> MAVDSAMELLFLDTFKHPSAEQSSHIDVVRFPCVVYINEVRVIPPGVRAHSSLPDNRAYGETSPHTFQLDLFFNNVSKPSAPVFDRLGSLEYDENTSIIFRPNSKVNTDGLVLRGWYNCLTLAIYGSVDRVISHDRDSPPPPPPPPPPPQPQPSLKRNPKHADGEKEDQFNGSPPRPQPRGPRTPPGPPPPDDDEDDPVPLPVSGDKEEDAPHREDYFEPISPDRNSVPQEGQYSDEGEVEEEQQEEGEEDEDDVDVEEEEDEDEDDRRTVDSIPEEEEEDEEEEGEEDEEGEGDDGYEQISSDEDGIADLERETFKYPNFDVEYTAEDLASVPPMTYDPYDRELVPLLYFSCPYKTTFEIEISRMKDQGPDKENSGAIEASVKLTELLDLYREDRGAKWVTALEEIPSLIIKGLSYLQLKNTKQDSLGQLVDWTMQALNLQVALRQPIALNVRQLKAGTKLVSSLAECGAQGVTGLLQAGVISGLFELLFADHVSSSLKLNAFKALDSVISMTEGMEAFLRGRQNEKSGYQKLLELILLDQTVRVVTAGSAILQKCHFYEVLSEIKRLGDHLAEKTSSLPNHSEPDHDTDAGLERTNPEYENEVEASMDMDLLESSNISEGEIERLINLLEEVFHLMETAPHTMIQQPVKSFPTMARITGPPERDDPYPVLFRYLHSHHFLELVTLLLSIPVTSAHPGVLQATKDVLKFLAQSQKGLLFFMSEYEATNLLIRALCHFYDQDEEEGLQSDGVIDDAFALWLQDSTQTLQCITELFSHFQRCTASEETDHSDLLGTLHNLYLITFNPVGRSAVGHVFSLEKNLQSLITLMEYYSKEALGDSKSKKSVAYNYACILILVVVQSSSDVQMLEQHAASLLKLCKADENNAKLQELGKWLEPLKNLRFEINCIPNLIEYVKQNIDNLMTPEGVGLTTALRVLCNVACPPPPVEGQQKDLKWNLAVIQLFSAEGMDTFIRVLQKLNSILTQPWRLHVNMGTTLHRVTTISMARCTLTLLKTMLTELLRGGSFEFKDMRVPSALVTLHMLLCSIPLSGRLDSDEQKIQNDIIDILLTFTQGVNEKLTISEETLANNTWSLMLKEVLSSILKVPEGFFSGLILLSELLPLPLPMQTTQVIEPHDISVALNTRKLWSMHLHVQAKLLQEIVRSFSGTTCQPIQHMLRRICVQLCDLASPTALLIMRTVLDLIVEDLQSTSEDKEKQYTSQTTRLLALLDALASHKACKLAILHLINGTIKGDERYAEIFQDLLALVRSPGDSVIRQQCVEYVTSILQSLCDQDIALILPSSSEGSISELEQLSNSLPNKELMTSICDCLLATLANSESSYNCLLTCVRTMMFLAEHDYGLFHLKSSLRKNSSALHSLLKRVVSTFSKDTGELASSFLEFMRQILNSDTIGCCGDDNGLMEVEGAHTSRTMSINAAELKQLLQSKEESPENLFLELEKLVLEHSKDDDNLDSLLDSVVGLKQMLESSGDPLPLSDQDVEPVLSAPESLQNLFNNRTAYVLADVMDDQLKSMWFTPFQAEEIDTDLDLVKVDLIELSEKCCSDFDLHSELERSFLSEPSSPGRTKTTKGFKLGKHKHETFITSSGKSEYIEPAKRAHVVPPPRGRGRGGFGQGIRPHDIFRQRKQNTSRPPSMHVDDFVAAESKEVVPQDGIPPPKRPLKVSQKISSRGGFSGNRGGRGAFHSQNRFFTPPASKGNYSRREGTRGSSWSAQNTPRGNYNESRGGQSNFNRGPLPPLRPLSSTGYRPSPRDRASRGRGGLGPSWASAN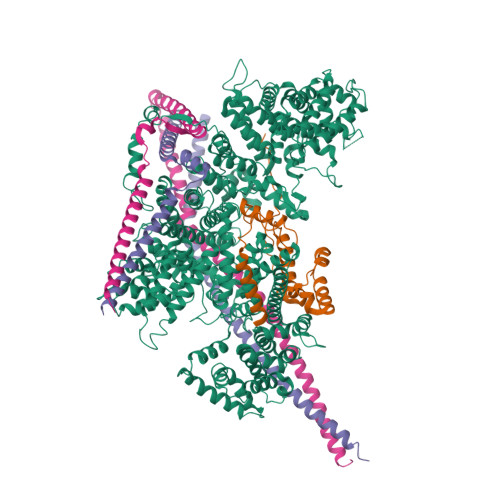SGSGGSRGKFVSGGSGRGRHVRSFTR;> PVATATATTVPATLAATTAAAATSFSTSAITISTSATPTNTTNNTFANEDSHRKCHRTRVEKVETPHVTIEDAQHRKPMDQKRSSSLGSNRSNRSHTSGRLRSPSNDSAHRSGDDQSGRKRVLHSGSRDREKTKSLEITGERKSRIDQLKRGEPSRSTSSDRQDSRSHSSRRSSPESDRQVHSRSGSFDSRDRLQERDRYEHDRERERERRDTRQREWDRDADKDWPRNRDRDRLRERERERERDKRRDLDRERERLISDSVERDRDRDRDRTFESSQIESVKRCEAKLEGEHERDLESTSRDSLALDKERMDKDLGSVQGFEETNKSERTESLEGDDESKLDDAHSLGSGAGEGYEPISDDELDEILAGDAEKREDQQDEEKMPDPLDVIDVDWSGLMPKHPKEPREPGAALLKFTPGAVMLRVGISKKLAGSELFAKVKETCQRLLEKPKDADNLFEHELGALNMAALLRKEERASLLSNLGPCCKALCFRRDSAIRKQLVKNEKGTIKQAYTSAPMVDNELLRLSLRLFKRKTTCHAPGHEKTEDNKLSQSSIQQELCVS;>[2x]MTNEEPLPKKVRLSETDFKVMARDELILRWKQYEAYVQALEGKYTDLNSNDVTGLRESEEKLKQQQQESARRENILVMRLATKEQEMQECTTQIQYLKQVQQPSVAQLRSTMVDPAINLFFLKMKGELEQTKDKLEQAQNELSAWKFTPDSQTGKKLMAKCRMLIQENQELGRQLSQGRIAQLEAELALQKKYSEELKSSQDELNDFIIQLDEEVEGMQSTILVLQQQLKETRQQLAQYQQQQSQASAPSTSRTTASEPVEQSEATSKDCSRLTNGPSNGSSSRQRTSGSGFHREGNTTEDDFPSSPGNGNKSSNSSEERTGRGGSGYVNQLSAGYESVDSPTGSENSLTHQSNDTDSSHDPQEEKAVSGKGNRTVGSRHVQNGLDSSVNVQGSVL>MAHNHRHKHADYKDDDDKKLNSATSADEQPHIGNYRLLKTIGKGNFAKVKLARHILTGKEVAVKIIDKTQLNSSSLQKLFREVRIMKVLNHPNIVKLFEVIETEKTLYLVMEYASGGEVFDYLVAHGRMKEKEARAKFRQIVSAVQYCHQKFIVHRDLKAENLLLDADMNIKIADFGFSNEFTFGNKLDTFCGSPPYAAPELFQGKKYDGPEVDVWSLGVILYTLVSGSLPFDGQNLKELRERVLRGKYRIPFYMSTDCENLLKKFLILNPSKRG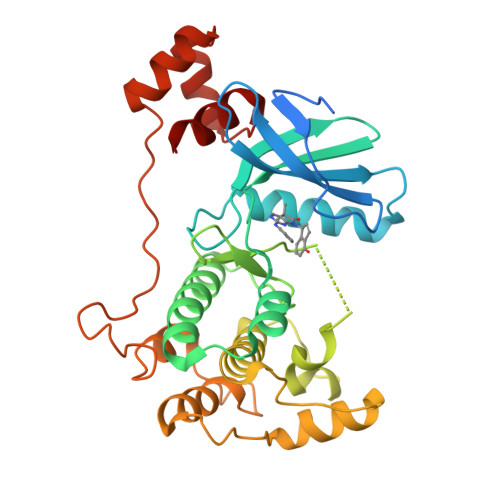TLEQIMKDRWMNVGHEDDELKPYVEPLPDYKDPRRTELMVSMGYTREEIQDSLVGQRYNEVMATYLLLGYK[2x]> MAKLTALTLLGMGLALFDRQKSSFQTRFNVHREVTPVELPNCNLVKGIDNGSEDLEILPNGLAFISSGLKYPGIMSFDPDKSGKILLMDLNEKEPAVSELEIIGNTLDISSFNPHGISTFIDDDNTVYLLVVNHPGSSST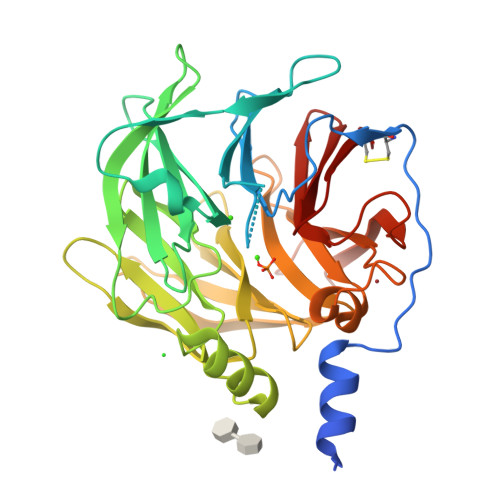VEVFKFQEEEKSLLHLKTIRHKLLPSVNDIVAVGPEHFYATNDHYFIDPYLQSWEMHLGLAWSFVTYYSPNDVRVVAEGFDFANGINISPDGKYVYIAELLAHKIHVYEKHANWTLTPLKVLSFDTLVDNISVDPVTGDLWVGCHPNGMRIFFYDAENPPGSEVLRIQDILSEEPKVTVVYAENGTVLQGSTVAAVYKGKLLIGTVFHKALYCDL>[3x]MQAQITGRPEWIWLALGTALMGLGTLYFLVKGMGVSDPDAKKFYAITTLVPAIAFTMYLSMLLGYGLTMVPFGGEQNPIYWARYADWLFTTPLLLLDLALLVDADQGTILALVGADGIMIGTGLVGALTKVYSYRFVWWAISTAAMLYILYVLFFGFTSKAESMRPEVASTFKVLRNVTVVLWSAYPVVWLIGSEGAGIVPLNIETLLFMVLDVSAKVGFGLILLRSRAIFGEAEA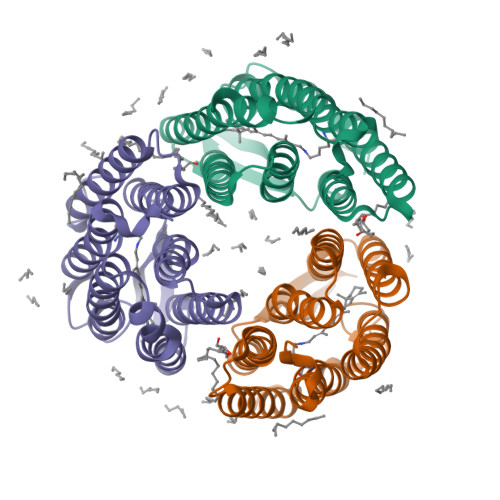PEPSAGDGAAATSDGSGIEGRSGAPHHHHHHHH> MSNQALYEKLEQTRTILSVKLAELINMTTIADRNDDDEGSFAQENSELAVATTSVMMVNNQTMQLIKNVQD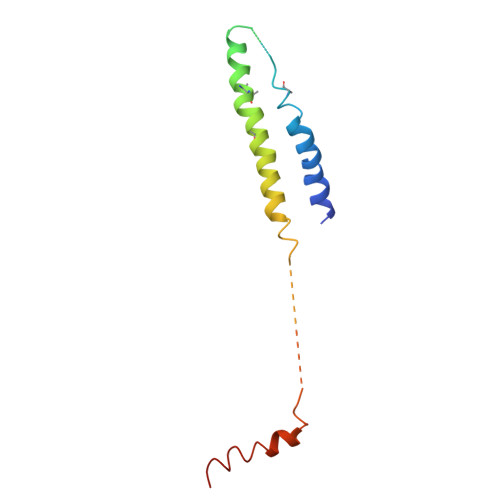LLILTRSIKEKWLLNQIPVTEHSKVTRFDEKQIEELLDNCIETFVAEKTT>MAHHHHHHMSLSDPTSTLMFAEAAEAADVVARQFSRNHATMETLAASLRAAPPPFVVTCARGSSDHAATYGKYLLETQLGLVVASASPSVGSVYAAPLQLRGALFIVISQSGKSPDLLRNAEAAKAAGARVIALVNVEDSPLAQLADTVIPLHAGAEKSVAATKSYLASLAALLQLAAYWKQDSSLRAALDLLPDALREAWQCDWSAVTEGLVEATNLFVLGRGLGLGAAQEAALKFKETCSLHAEAYSSAEVKHGPMALV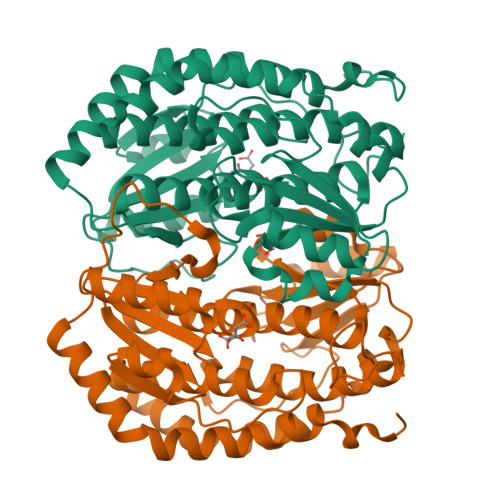DRGFPVLAFAQPDETGAGTRAVVEEFTARGAQVWMAGAGGNLPVAAAPHPLCAPLLTVQSFYRAINALALRRGFNPDLPPHLNKVTETV[2x]>ATMKYVGSIDQGTTSTRFIIFDERQRPVSVHQVPHTQHTPHPGWLEHDPMEIFRSACKCMSVAIAKLRQKDASFRKIEAIGITNQRETTVAWDRVTKEPLCYAPVWNDLRTYDITKKVTAELGGGDSMFASKITGLPVSTYFAAFKMRWMLENVPAVADACRRGTLCFGTIDTWLMYKLSGGKAFVTDVTNASRTFLMDLRTRKWSPELCEKLKIPMETLPEIRSNSELFGYVETDECGVAAALNERTPIMGSIGDQQSALFGNMCFEKGEAKNTYGTGCFLLMNVGEEARFSKHGLLSTVGFQVGRDGPCYYALEGAIACAGATVEWMRRNMNLFSHITECEKLARSVPGTQGIVFVPAFSGLLAPYWDPSARGTIVGMTLKTTRAHVIRAALQAIALQLNDVVGSMKRDAGLNLSSLRVDGGLSKNGLLMEIQASLLGVDILVPSMHETTALGAALCAGLAAGVWTSLEEVKAVSRRENSWK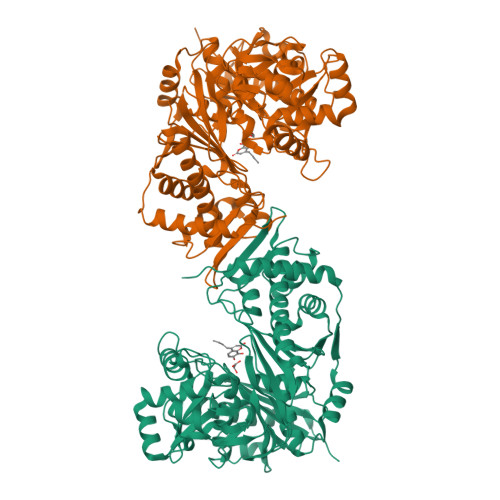TVSPSGSAMEREAMIAEWREALKRTKWAKL[4x]>MSKPQPIAAANWKCNGSQQSLSELIDLFNSTSINHDVQCVVASTFVHLAMTKERLSHPKFVIAAQNAIAKSGAFTGEVSLPILKDFGVNWIVLGHSERRAYYGETNEIVADKVAAAVASGFMVIACIGETLQERESGRTAVVVLTQIAAIAKKLKKADWAKVVIAYEPVWAAGTGKVATPQQAQEAHALIRSWVSSKIGADVAGELRILYG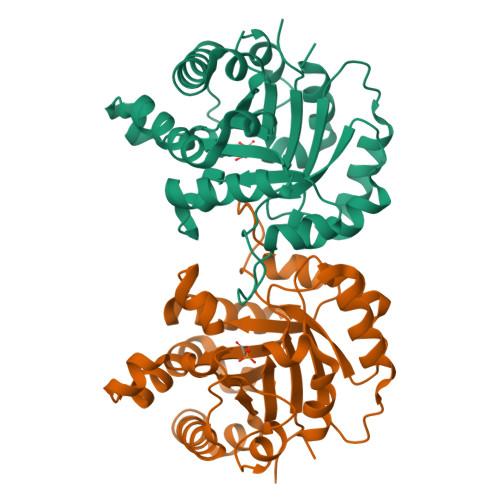GSVNGKNARTLYQQRDVNGFLVGGASLKPEFVDIIKATQ[4x]N-(cyclohexylmethyl)-4-oxo-4H-1-benzopyran-2-carboxamide | C17 H19 N O3 | 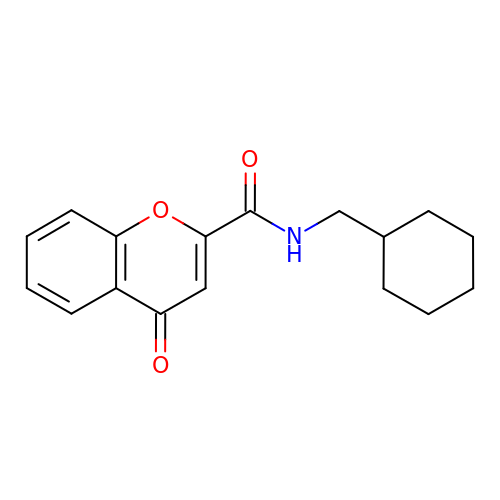ZNVNVRHEGZKDAE-UHFFFAOYSA-N>MTQTAPAAVAYSVNHAGVAAIVLDRPEASNALDRTMKTELLQALLAAGGDPAVRAVVMSAAGKNFCVGQDLAEHVEALRDDPAHAMDTVREHYNPVLEALDAIKVPVVVAINGACVGAGLGLALGADIRIAGQRAK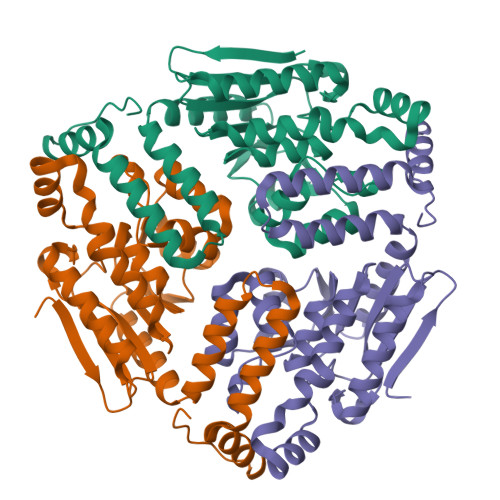FGTAFTGIGLAADSALSASLPRLIGASRATAMFLLGDTIDAPTAHTWGLVHEVVDEGSPADVANSVAGRLAGGPTAAFSEVKELLRRNAVAPLGDVLEREASAQQRLGASRDHSAAVEAFLAKDKPVFVGR[3x]>MKFTLLSVVAIAAAASDSYAAPAASSLAGPVTTGVFSAVSAIPSFATNLSGQVASATSTVLSGSTASGSSATAAPSASASGASSMQSMASSLSGSAFSPSSMMPIASGNMTMPNMTSSASASSAASTATGVAGGAGSNSSSSCAPTSLPASATELPTTVPTGTVITGDYTGSYRPQVHYSPPKGFMNAPNGCHRDRNGTYHLYYQYNPLEYVAGNQHWGHATSDDLYHWTNQPIAIFPPNSTSQVFSGSAVLDPNNTSGFFPNTTDGVVAVYTLNTPTLQVQEVAYSTDGGYNFTPYENNPVLSVGSNQFRDPKVFWYEDHWVMAVAAANDFTIEIYTSPNLTSWTFASNFTHHGLLGLAYECPNLVQVPFQDDPSKSAWLMYISINPGAPLGGSVGQYFPGDFNGTHFVAYDSAARIADFAKDNYASQWFADTENGESISIAWASNWQYTQQVPTSAQAFRSAMSLPRRNYLTNITRLGWDLVSLPYDLSPVVGPSLLSSSEANSTADVDFTNVTSNAVWFSLNVTLPDAAIQNASLISADASINITFLPSTKCSSSSGSGSDSPAATLTYFYAGLTNGALALTRPAASSSWGAENPFFTDKFSYTLVDPLTSLVGVFDRS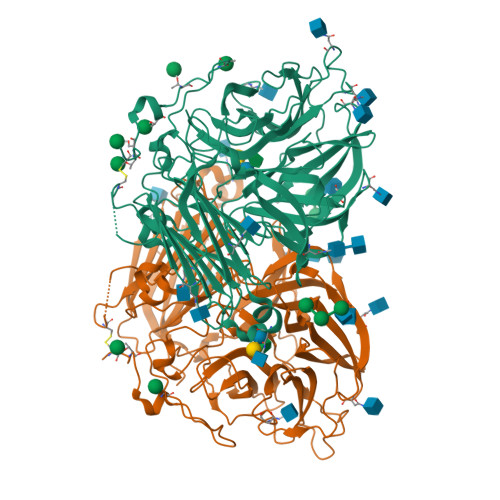MLEVFVNEGAHSATMLVFPDSPVGSMKVATGGLPEGTQVNLQVNGLESTWQSS[4x]> ADS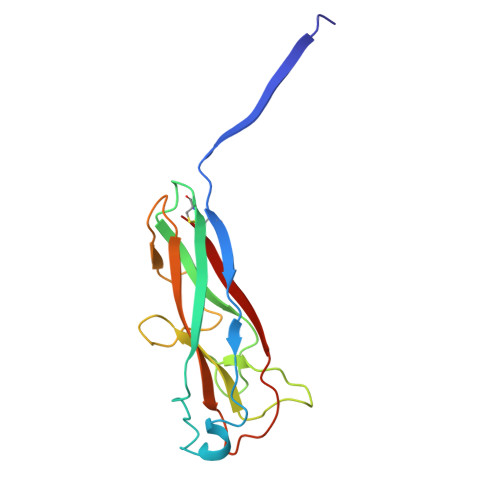TITIRGYVRDNGCSVAAESTNFTVDLMENAAKQFNNIGATTPVVPFRILLSPCGNAVSAVKVGFTGVADSHNANLLALENTVSAAAGLGIQLLNEQQNQIPLNAPSSALSWTTLTPGKPNTLNFYARLMATQVPVTAGHINATATFTLEYQ> 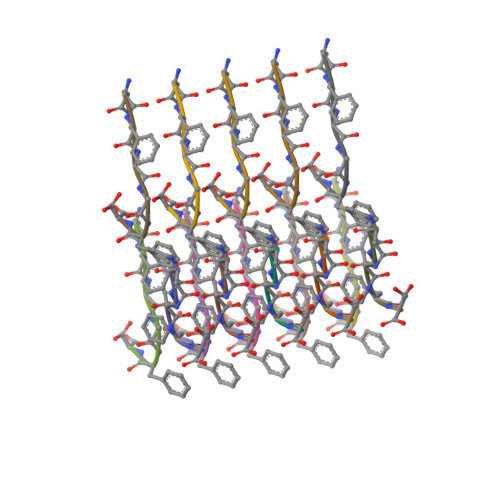NFGAFS> MLDRFATKQTQEKLKIGVVGTFAIGCLFPLLSDFKRSYPHIDLHISTHNNRVDPAAEGLDYTIRYGGGAWHDTDAQYLCSALMSPLCSPTLASQIQTPADILKFPLLRSYRRDEWALWMQTVGEAPPSPTHNVMVFDSSVTMLE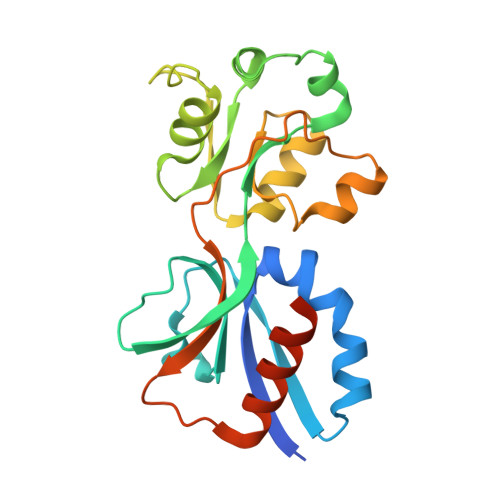AAQAGMGVAIAPVRMFTHLLSSERIVQPFLTQIDLGSYWITRLQSRPETPAMREFSRWLTGVLHKTSGSHHHHHH>[4x]GPLGSMTKYTYPATLLCDFYKVSHKEQYPEGTELIYSTWTPRTSRVEDIDRVVAFGFQGFIKKYLIDYFNENFFKRPKQDVVNEYKRVIKHTLQVDDPDASHIESLHELGYLPIKIKAVKEGTFIPIKVPMLTIENTIPEFFWITNYLETLMSNEIWQPTTSATLAYEYRKILDEYAMETVGNKLAVDFQGHDFSMRGMSSLESTKLSG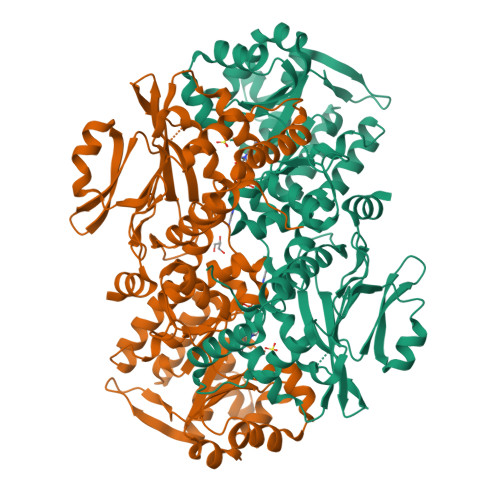AGHLLSFTGTDTIPAILYHEEFYNANIENELVGSSIPATEHSVMCANGQDEYVVFKKLITETYPEGFVSIVSDTWDFWNVIDTVVRKLKGDILKRDGKVVIRPDSGDPVKIICGDPEAKDELVRKGLIEVLWDIFGGNVTDKGYKVLDPHIGAIYGDAITISRCKEICKKLAAKGFASVNVVFGIGSFTYQYNTRDTFGFAMKATYTVVNGEERQIFKNPKTDDGTKKSQKGLVAVVNNGNELSLVDELDRNAYKQLSNDDILEDVFINGQLLRNQTLSEIRELLLD>[2x]MNPAAEAEFNILLATDSYKVTHYKQYPPNTSKVYSYFECREKKTENSKLRKVKYEETVFYGLQYILNKYLKGKVVTKEKIQEAKDVYKEHFQDDVFNEKGWNYILEKYDGHLPIEIKAVPEGFVIPRGNVLFTVENTDPECYWLT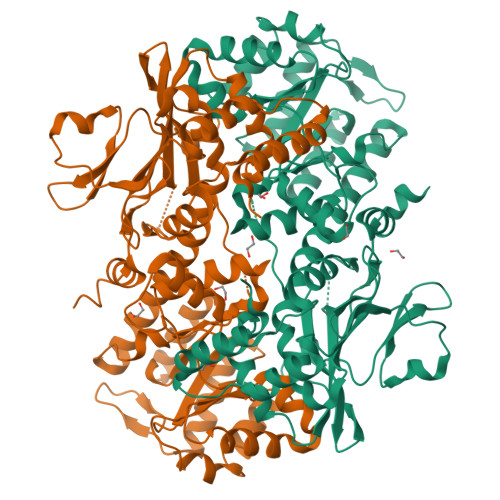NWIETILVQSWYPITVATNFREQKKILAKYLLETSGNLDGLEYKLHDFGYRGVSSQETAGIGASAHLVNFKGTDTVAGLALIKKYYGTKDPVPGYSVPAAEHSTITAWGKDHEKDAFEHIVTQFSSVPVSVVSDSYDIYNACEKIWGEDLRHLIVSRSTQAPLIIRPDSGNPLDTVLKVLEILGKKFPVTENSKGYKLLPPYLRVIQGDGVDINTLQEIVEGMKQKMWSIENIAFGSGGGLLQKLTRDLLNCSFKCSYVVTNGLGINVFKDPVADPNKRSKKGRLSLHRTPAGNFVTLEEGKGDLEEYGQDLLHTVFKNGKVTKSYSFDEIRKNAQLNIELEAAHHLEHHHHHHHH(6E,10R,13S,18E)-2,6,10,15,19,23-hexamethyltetracosa-2,6,10,11,13,14,18,22-octaene 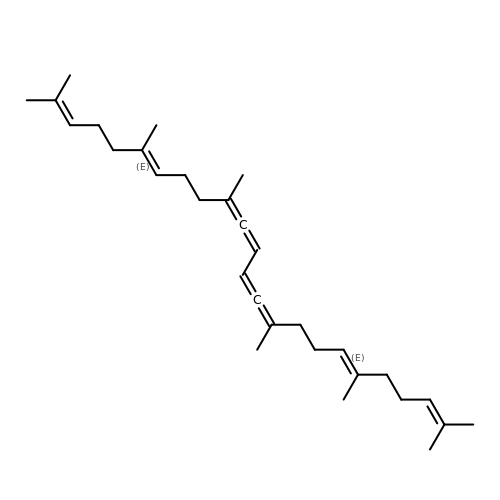| C30 H46 | PALVLARMLPXARO-HCTXVGCHSA-N>AKHTLLRHEGIETVSYATQSLVVANGGLGNGVSRNQLLPVLEKCGLVDALLMPPNKPYSFARYRTTEESKRAYVTLNGKEVVDDLGQKITLYLNFVEKVQWKELRPQALPPGLMVVEEIISSEEEKMLLESVDWTEDTDNQNSQKSLKHRRVKHFGYEFHYENNNVDKDKPLSGGLPDICESFLEKWLRKGYIKHKPDQMTINQYEPGQGIPAHIDTHSAFEDEIVSLSLGSEIVMDFKHPDGIAVPVMLPRRSLLVMTGESRYLWTHGITCRKFDTVQASESLKSGIITSDVG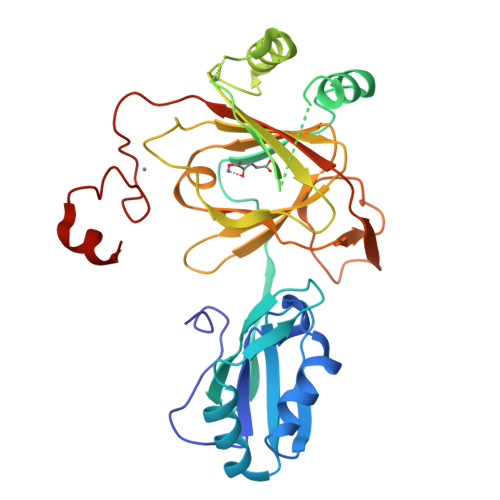DLTLSKRGLRTSFTFRKVRQTPCNCSYPLVCDSQRKENLYFQGLEHHHHHH[4x]>GDTPPGNVQSTFKKMYP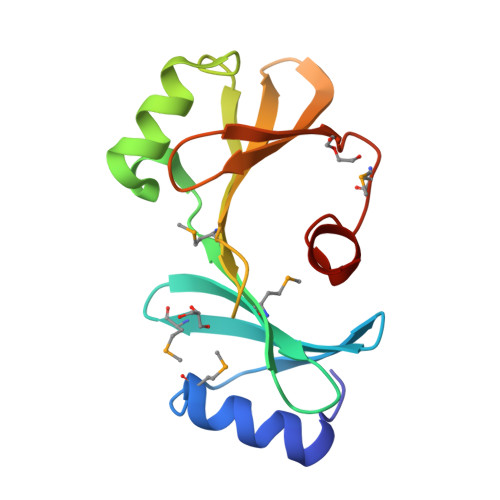KANGVAWSQDDGYYCANFAMNGFTKNVWFNVRGQWVMTLTDLVSLDRLTPTVYNAFVSGPYANWVVDNVTMVEFPKWQAIIVIKVGQDNVDIKYQLFYTPQGILLKTRNVSDMYDILGPSTFLAN[2x]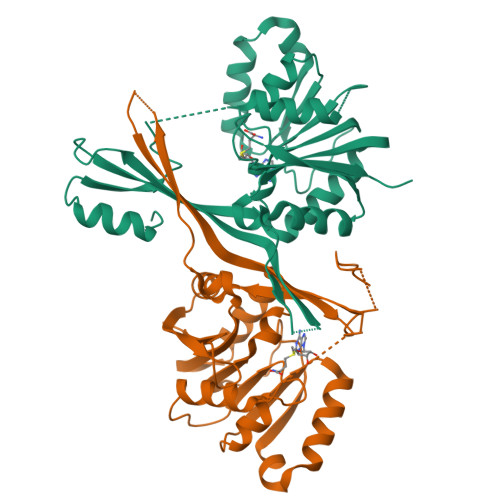>[2x]MGSSHHHHHHSGGLVPRGSMSNQLERGPVRTPHADVLLASVGERGVLCDFYDEGAADTYRDLIQDADGTSEAREFATRTGPVSGPVLELAAGMGRLTFPFLDLGWEVTALELSTSVLAAFRKRLAEAPADVRDRCTLVQGDMSAFALDKRFGTVVISSGSINELDEADRRGLYASVREHLEPGGKFLLSLAMSEAAESEPLERKQELPGRSGRRYVLHVRHLPAEEIQEITIHPADETTDPFVVCTHRRRLLAPDQVVRELVRSGFDVIAQTPFASGGAGRKDMVLVEAVMPGATADAR MreB is a bacterial protein belonging to the actin superfamily. This protein polymerizes into an antiparallel double-stranded filament that determines cell shape by maintaining cell wall synthesis. Here, we studied MreB3 and MreB5 in Spiroplasma eriocheiris (SpeMreB3 and SpeMreB5, respectively), a model organism for studying Spiroplasma swimming. SpeMreB3 adopts a canonical actin fold composed of four subdomains (IA, IB, IIA and IIB) and consists of the same secondary structure elements as CcMreB, Thermotoga maritima (Tm) MreB and SciMreB5, except for the C-terminal region.

The crystal structures of nucleotide-free (Nf) SpeMreB3 and its AMPPNP complex were determined at 1.90 and 1.75 Å resolution. The Nf-SpeMreB3 crystal belongs to the space group P21 and contains a single molecule in an asymmetric unit. Nf-SpeMreB3 forms protofilaments along the crystal a axis in the P21 crystal. Thus, the protofilaments are arranged in an antiparallel manner. The interaction between IIA and IB' (with and without a prime indicating i and i-1 subunits, respectively), which has been observed in CcMreB, TmMreB and SciMreB5 protofilaments, is not found in the Nf-SpeMreB3 protofilament, whereas the IIA-IIB' interaction is conserved in Nf-SpeMreB3. This IIA-IIB’ interaction is mediated by a hydrogen-bonding network and is stabilized by an electrostatic interaction between E285 and the N-terminal end of the α-helix starting from V216'. Nf-SpeMreB3 had larger ω1 and φ values than SpeMreB3-AMPPNP complex Mol-A (4.6° and 3.5°, respectively), showing a wider nucleotide-binding cleft and a more uneven overall conformation. While our Nf-SpeMreB3 crystal structure forms a protofilament, we suppose that ATP binding is necessary to polymerize SpeMreB3, since filaments were not observed in the absence of nucleotides under solution conditions. Although some intra-protofilament interactions along the filament axis were observed in Nf-SpeMreB3, the interaction area is smaller than that in SpeMreB3-AMPPNP. This difference is derived from domain closure upon AMPPNP binding, suggesting that this conformational change is necessary to form filaments in solution.

> GSHMTITDVLKNTFNISPKPPRKFIAIDLGTTNSIAYIGGRGIIYNEASVMAYETGTKKLVALGEDARKLIGKTHDKIEIYTPLRNGAITDLRIAEEFIQHIGNRAKVQDVWKGSIVLIACPKSVTELERRAMVEMCKHLGADLVQVEEDTLMAALGAGANIFAPKGTFILDIGGGKTSAGIISAGGIVVSKSIKIAGNYIDEEILKYIRAKHTISIGVVTAEQIKKQIGSLYKGKETKKMVIFGRDVVTGMPKETEILDSEIRKLLISIFSSITQLVTDILESTPAELAGDAVMNGLLVSGGCAQISGLKEFLESYFQIPVKIAKNPQTAVIDGCIAYEKEIRDRLIEENKKNK> MVNTEEDGLPRLIDAIEEASKIPAKRRQTPIKPTIEKLTTHLYTHGASPDSLLRLADLLTLRNHLDQASLAAITRNLYPSSTVSDEVVLRFIGALGHGQLKPTLALQALFLRWLVMVYHLLENPGVLGQVYGVLFDLLDTAAIRPQLCHLLALVTRRKHVRPFRIQAILTLSRQTG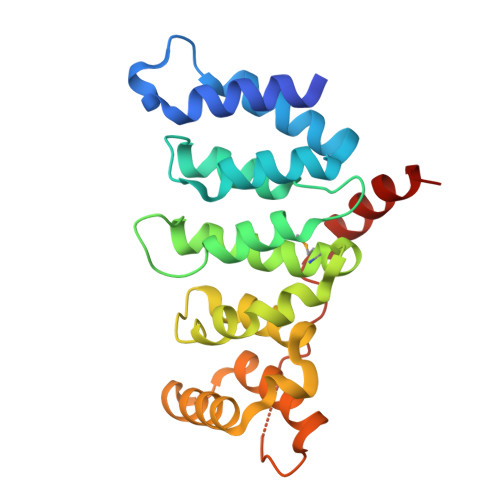GDPNLTGLLRVFKNYYPEIIVGDATKGRASAFKHPDPQWRQHLDEIQQRRSEA>MFKVYGYDSNIHKCVYCDNAKRLLTVKKQPFEFINIMPEKGVFDDEKIAELLTKLGRDTQIGLTMPQVFAPDGSHIGGFDQL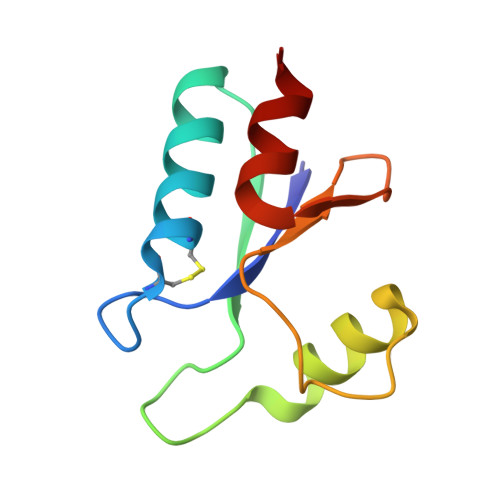REYFK[2x]> MERKISRIHLVSEPSITHFLQVSWEKTLESGFVITLTDGHSAWTGTVSESE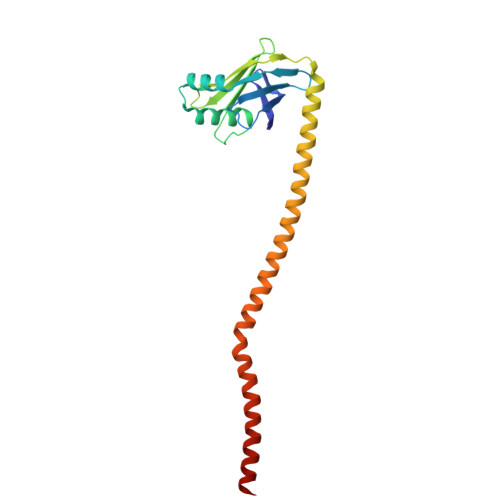ISQEADDMEMEKGKYVGELRKALLSGAGPADVYTFNFSKESCYFFFEKNLKDVSFRLGSFNLEKVENPAEVIRELICYCLDTTAENQAKNEHLQKENERLLRDWNDVQGRFEKCVSAKEALETDLYKRFILVLNEKKTKIRSLHNKLLNAAQ> MGSHHHHHHHHENLYFQSVSGETPLEIAVSLGLGWNLGNQLDAHNNGVADETSWGNAAATQALFDALANAGFTSVRIPVTWLGHVGEAPDYTIDETYLNRVAEVVGYAESAGLNAIINIHHDGANSQYWLDIKDAATDETVNSAVKAQLAAMWTQIANRFADKGNFLVFEAMNEIHDGSWGWGDNRTDGGRQYAVLNEWNQVFVDAVRATGGNNQTRYLGVPGYVTNIDLTVENFVLPQDVVDNRLMVAVHFYDPIDYTENADNIYSQWGHTADPSLKADWGDEDNVTGQFAKM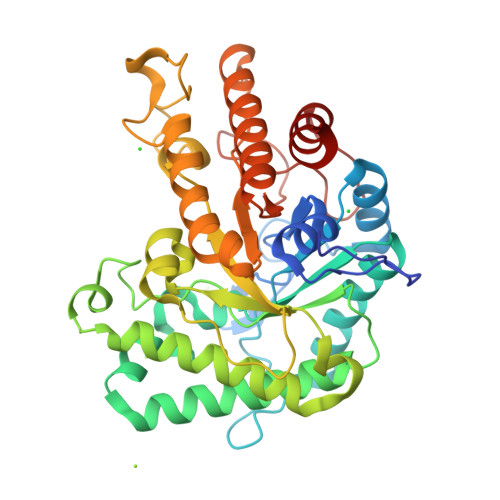KETFIDQGIPAYIGEMGCVHRADDLSESFRLYYLEYVCKAAKDYGMPPFYWDAGGDGTGTQSWALFNHATGEMLNNAQEVIDVMKRGIFTV> MHHHHHHHAVRASEISRVYEAYPEKKATLYFLVLGFLALIVGSLFGPFQALNYGNVDAYPLLKRLLPFVQSYYQGLTLHGVLNAIVFTQLFAQAIMVYLPARELNMRPNMGLMWLSWWMAFIGLVVAALPLLANEATVLYTFYPPLKGHWAFYLGASVFVLSTWVSIYIVLDLWRRWKAANPGKVTPLVTYMAVVFWLMWFLASLGLVLEAVLFLLPWSFGLVEGVDPLVARTLFWWTGHPIVYFWLLPAYAIIYTILPKQAGGKLVSDPMARLAFLLFLLLSTPVGFHHQFADPGIDPTWKMIHSVLTLFVAVPSLMTAFTVAASLEFAGRLRGGRGLFGWIRALPWDNPAFVAPVLGLLGFIPGGAGGIVNASFTLDYVVHNTA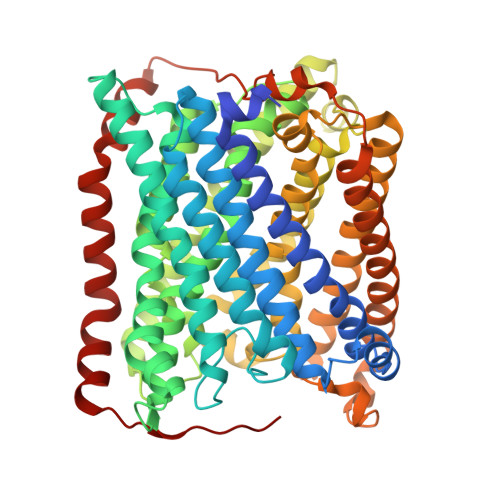WVPGHFHLQVASLVTLTAMGSLYWLLPNLTGKPISDAQRRLGLAVVWLWFLGMMIMAVGLHWAGLLNVPRRAYIAQVPDAYPHAAVPMVFNVLAGIVLLVALLLFIYGLFSVLLSRERKPELAEAPLPFAEVISGPEDRRLVLAMDRIGFWFAVAAILVVLAYGPTLVQLFGHLNPVPGWRLW>SNMREIAPKEFVLDMGAGWNLGNAMDTYNSDE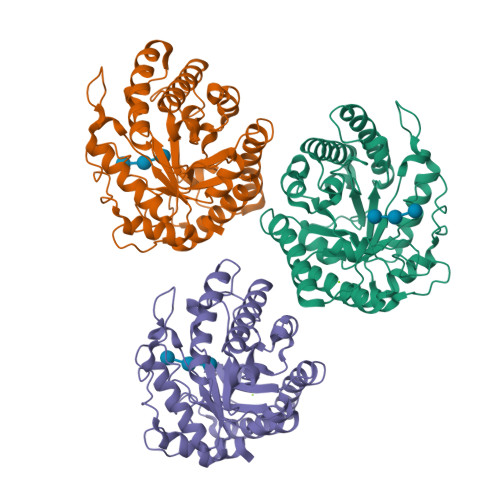TAWGNPLTTKAMIDEIAKMGFKTLRLPVTWKFHIGEGPDYLIEANWLDKVEAIANFALENEMYVIINIHHDETWILPTYEKADEVKDELSKVWTQIANRFKTYGDYLIFETLNEPRHKGTPEEWKGGTQEGRDAVNQYHQVSVDAIRATGGNNAKRKIMVSTYAASTASNALNDYLVPNGDKNVIVSVHSYFPYQFCLDGTDSTWGTEADKTALLAELDKIRDKFIVEDNRAVVMGSWGSTFSDNPEDRLAHAEFYARACAERGICPIWWDNGNVDEFGIFNRNTLEWNYPEIAEAIVK[3x]> MEVNEKAPAQARPTVFRWTGGGKEVYLSGSFNNWSKLPLTRDQNNFVAILDLPEGEHQYKFFVDGQWTH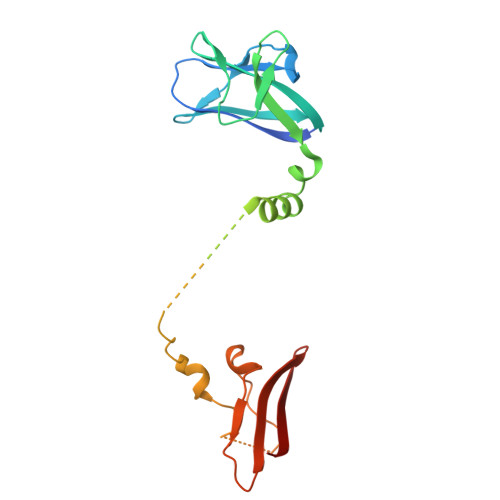DPSEPIVTSQLGTVNNIIQVKKTDFEVFDALMVDSQKCSDVSELSSSPPGPYHQEPYISKPEERFKAPPILPPHLLQVILNKDTGISCDPALLPEPNHVMLNHLYALSIKDGVMVLSATHRYKKKYVTTLLYKPI>GPMEEAPFYRDTWVEVDLDAIYNNVTHIKEFIPSDVEIFAVVKGNAYGHDYVPVAKIALEAGATRLAVAFLDEALVLRRAGITAPILVLGPSPPRDINVAAENDVALTVFQKEWVDEAIKLWDGSSTMKYHINF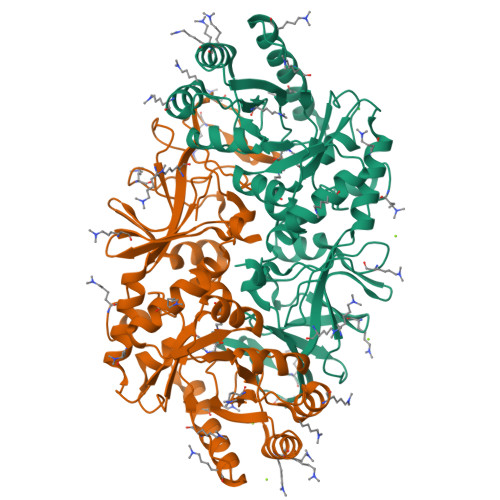DSGMGRIGIRERKELKGFLKSLEGAPFLELEGVYTHFATADEVETSYFDKQYNTFLEQLSWLKEFGVDPKFVHTANSAATLRFQGITFNAVRIGIAMYGLSPSVEIRPFLPFKLEPALSLHTKVAHIKQVIKGDGISYNVTYRTKTEEWIATVAIGYADGWLRRLQGFEVLVNGKRVPIVGRVTMDQFMIHLPCEVPLGTKVTLIGRQGDEYISATEVAEYSGTINYEIITTISFRVPRIFIRNGKVVEVINYLNDI[2x]> SEFELMKRLSEIKVLPILESLKYIKHNHASVVRFGDGEIDLMTGHSIPYQDYNEKLAKRLQQILQTKSDEKLLVCLPDVFSNMDRYNQNARHFWERHFLKYSEFYLNCCDAPFYGSTFISRPYIDLID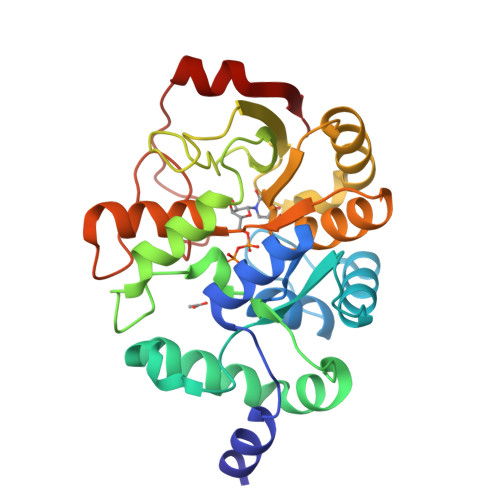KSPSEAYFESLKELWRGKDLLIVEGATSRSGVGNDLFVAASSIKRLVCPSKNAFQYYDEILRLTEKNAKNRLILVMLGPTAKVLVADLTTKGYQAIDLGHIDSEYEWYEMGATYKVKLTNKHTAEFNYDEGIELEFSQEYQEQIVARIG> MPCSCASGCQKSKNGGSTPSIRDHVADYYGKTLQSSADLKTSACKLAAAVPESHRKILADIADEVLEKFYGAGSTLPADGSLEGATVLDLGCGTGRDVYLASKLVGEHGKVIGVDMLDNQLEVARKYVEYHAEKFFGSPSRSNVRFLKGFIENLATAEPEGVPDSSVDIVISNCVCNLSTNKLALFKEIHRVLRDGGELYFSDVYADRRLSEAAQQDPILYGECLGGALYLEDFRRLVAEAGFRDVRLVSVGPVDVSDPQLRKLVPDVQFYSCTFRCFKVATLE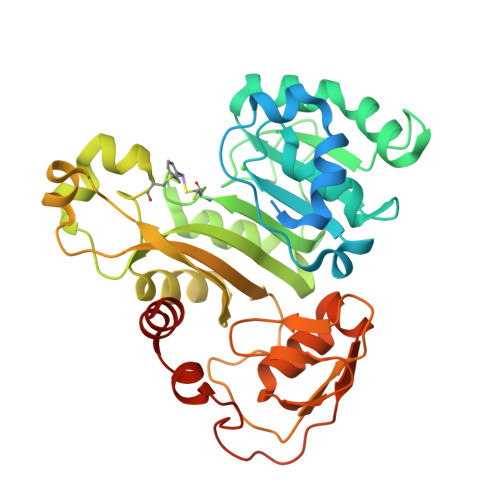ATREDYGQSATYLGGIGEEFKLDRFFTFPREKPVRVDRNTAEIIRHSRLHQWFSVSAEQQHMGLFKANDSYALLHAPLSMQVEQLVSHHHHHH> MKHHHHHHPMSDSKTVNYFDIITIKHQDTDAFLHSHLARYPQRYEDGRISSAGQQVTGYTHPDFNNQWEVLPPHGSDVGKGQAVLLNQHIRLRHVATDTYLLAHDVASPFYPTNEEITTVTLEEGDGELYPETLFAFQPLKKSDEGHVLKSKTVSFRLFHVDTSVALWTHNDELLPDWGFQQQEINGNKKVIDPSNNWVVDEIVNLDEVRKVYIPKVVKPLP

Protein O-mannosyltransferases (PMTs) are conserved endoplasmic reticulum membrane-embedded enzymes responsible for the transfer of mannose from dolichol phosphate-mannose (Dol-P-Man) to serine/threonine-rich protein substrates or unfolded proteins. PMTs from three subfamilies form obligate dimers with different substrate specificities and require the concerted action of their transmembrane domains (TMDs) and a luminal MIR domain for catalysis. Here, we present structures, native mass spectrometry, and structure-based mutagenesis of the fungal Pmt4 homodimer. The core fold of the TMDs and MIR domain is conserved with the Pmt1-Pmt2 heterodimer, indicating a shared catalytic mechanism.

Therefore, in order to be able to compare PMT2 and PMT4 family MIR domains from the same species, we additionally purified the scPmt4-MIR domain and solved the crystal structure to 1.3 Å resolution. Aside from minor conformational differences in the β4−β5 and β8−β9 loops, the scPmt4- and ctPmt4-MIR domain structures are highly similar (RMSD 0.87 Å over 194 Cα-atoms) and comprise the characteristic peculiar β-trefoil fold i.e. six β-hairpins arranged within a pseudo-threefold symmetry (three MIR-motifs: MIRm1,2,3), altogether forming a β-barrel and a triangular cap. Overall, the scPmt4-MIR domain closely resembles scPmt2 in its core fold (RMSD 1.38 Å over 168 Cα-atoms) and accordingly putative binding sites for O-mannosylated peptides could also be located in each MIR-motif (α, β, γ and δ). Interestingly, whilst in the scPmt2-MIR the sugar-binding γ site of MIRm3 is sterically blocked, the γ site within the scPmt4-MIR is open and comprises a LWTH motif more similar to the α and β sites. Characteristically, the Pmt4-MIR domain structures reveal a unique β-hairpin insertion (β-ins) of seven residues (RY(D/E)(D/N)GRΦ) in β2−β3 of MIRm1. β-ins is extensively stabilised by internal hydrogen-bonding and a central salt-bridge between the conserved 4th and 6th residue (ct: D370:R372, sc: D364:R366). It is fixed on top of the cap scaffold by hydrogen-bonding of the tyrosine (ct: Y368, sc: Y362) to a glutamate (ct: E441, sc: E434), and of the centrally-fixed arginine to the mainchain around a proline (ct: P434, sc: P427) within MIRm2. To assess the importance of β-ins on the O-mannosyltransferase activity of Pmt4 in vivo, yeast strains were created that express either FLAG-tagged wild-type or mutated scPmt4 (scPmt4-FLAG), specifically with a deletion of β-ins (Δ362-368) or alanine substitutions of residues crucial for stabilising its fold (Y362A/D364A/R366 A (YxDxR), P427A/P430A (PP) and W496A). Consistent with the temperature-sensitive growth phenotype, the glycosylation pattern of Ccw5 isolated from yeast strains expressing scPmt4 β-ins mutant proteins Δ362-368, YxDxR and W496A is very similar to that of the null mutant pmt4, demonstrating that the enzyme function is largely lost in vivo.> MATQFDENTVITIFGASGDLSKKKTFPALFGLYREGYLNPTTKIIGYARSKLSNEDLREKVKPFLKKPNGAKDDAKVNEFLSMVSYHAGPYDSDEGYLELKKIIEEFEAEKKVDEPHRLFYLALPPSIFIDVCSKLKENLYTESGIQRVIVEKPFGHDLQSATELQEKLAPLFSEDELFRIDHYLGKEMVKNLLLMRFGNTFLNAAWNKENIQSVQVVFKEPFGTEGRGGYFDSIGIIRDVMQNHLLQVLTLLTMERPVSFDPESVRDEKVKVLKAFSPIDHDDILIGQYGRSVDGSKPSYLDDETVKEDSKCVTFAAIGFKIANERWDGVPIVMRAGKALNEGKVEIRIQFRRVASGMFTDI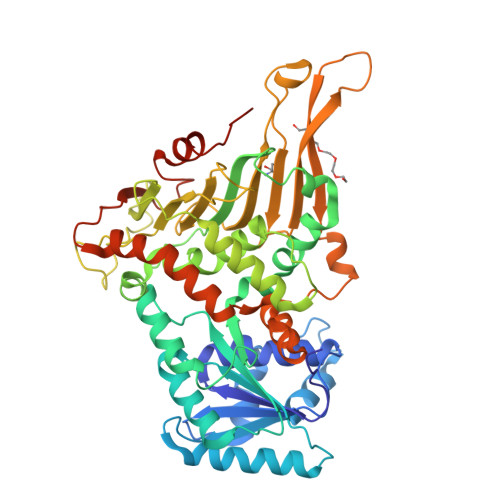PNNELVIRIQPNEAIYLKCNAKTPGLANENQTTELDLTYSERYKNYWIPEAYESLIRDALLGDHSNFVRDDELDVSWKLFTPLLNYLEGPDGPQPKIYPYGCRSPDGLVEFLADHGYTFSKPGSYQWPVTTPKM> TGAGDRHNLKTEWPELVGKSVEEAKKVILQDKPEAQIIVLPVGTIVTMEYRIDRVRLFVDKLDNIAQVPR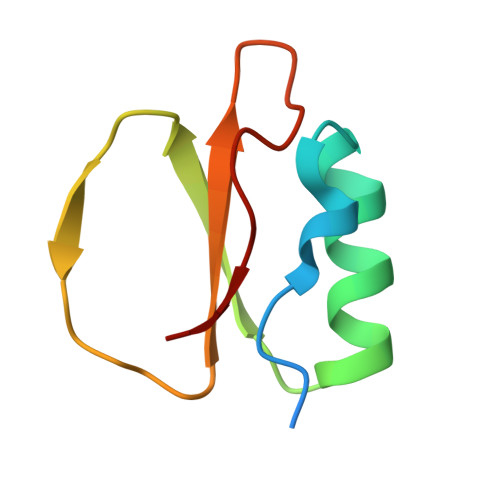VG>MAHHHHHHSLTNFSQQHLPLVEKVMVDFIAEYTENERLKEAMLYSIHAGGKRLRPLLVLTTVAAFQKEMETQDYQVAASLEMIHTYSLIHDDLPAMDDDDLRRGKPTNHKVFGEATAILAGDGLLTGAFQLLSLSQLGLSEKVLLMQQLAKAAGNQGMVSGQMGDIEGEKVSLTLEELAAVHEKKTGALIEFALIAGGVLANQ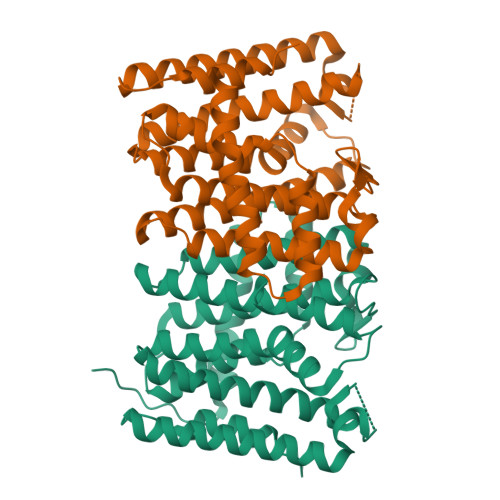TEEVIGLLTQFAHHYGLAFQIRDDLLDATSTEADLGKKVGRDEALNKSTYPALLGIAGAKDALTHQLAEGSAVLEKIKANVPNFSEEHLANLLTQLQLR[2x]>MELR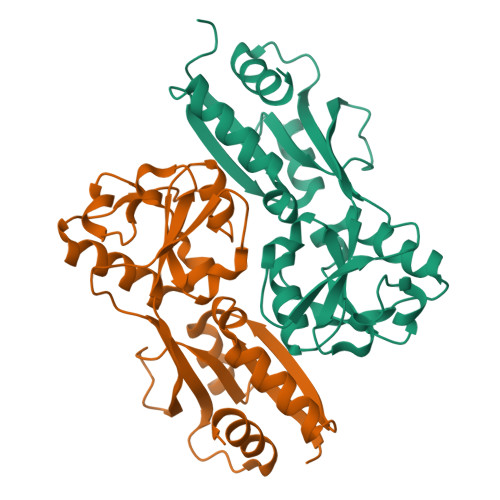HIRYFLAVAEERHFTRAAARLGIGQPPLSQQIKDLERELGALLFRRVSYGAELTEAGIAFLDVVKEIPVMAERATQAAQRAVRGELGVLRVGFTASSAFNSVVPTAIRAFRRAYPDVRLQLEEDNTTRLADGLNEGSLDVAFLRPGFAGSERFHLRMLSEEPMMIVMAENHPAASYEEISLSAFRDETFLLFPREIGLTLYDSVIESCRTAGFEPTIGQLAPQIASVINLVAAEMGVSIVPASMSQVKVIGVVYRHIADQTPTAKLALAYRRGDTSPVLRNFVLTVFP[8x]>MSPFKKTYVLKLYVAGNTPNSVRALKMLKNILEQEFQGVYALKVIDVLKNPQLAEEDKILATPTLAKILPPPVRKIIGDLSDREKVLIGLDLLYDEIREREAE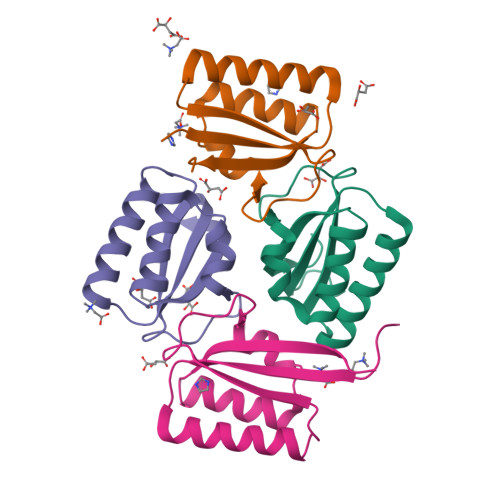DQ[4x]>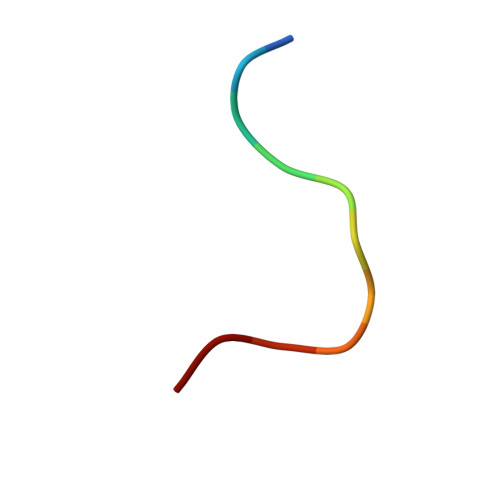 KLKLLVVIRLK>[3x]MTAPIPVVPVSRPQAKTSLKLPNNQVWVTRK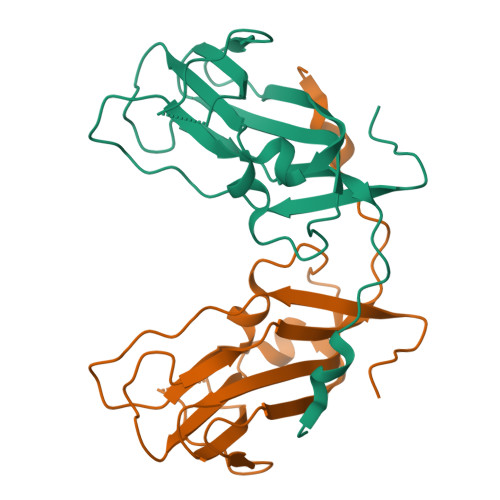ASEWSAKTIDTNDAIPFKTIVEGIPEINSETKFYRLLIGFVAVSDGTFGMVDGVTGDVIPDPPVVGRLGFKKNTYRSRDFDLGGKLLNQLDDRAIVWCLDERRRDAKRVQLAGYWIAISKPAPLMPPEDFLVNQD Here we characterize a metal-dependent, bifunctional isoprenyl diphosphate synthase from the leaf beetle Phaedon cochleariae by structural and functional analyses. Isoprenyl diphosphate synthase in P. cochleariae (PcIDS1, EC 2.5.1.1) produces FPP in the presence of Mg2+, but preferably forms GPP when exposed to the heavy metal ions (HMIs) Co2+ or Mn2+. Inter- and intramolecular cooperative effects in the homodimer strongly depend on the provided metal ions and regulate the biosynthetic flux of terpene precursors to either biological defence or physiological development. Strikingly, a unique chain length determination domain adapts to form geranyl or farnesyl pyrophosphate by altering enzyme symmetry and ligand affinity between both subunits.

Stabilized by cation–π interactions with R427, the F315 side chain positions IPPHAl for nucleophilic attack. V286 and I420 form the bottom of this specificity pocket and act as a molecular ruler, whereas F282 and F315 engage in π-stacking with both allyl groups.

>[2x]GSFSKEESREFMAIFPDIVRDLTDAGRHTDIPEVTKRFAKVLQYNVPTGKKTRGLSTVIAYKMLEKPENLTPENVRLAGILGWCVELLQASLLIMDDLMDRSETRRGQPCWYRQENVGFLAINDCLHVESSLYSVLRKYFSHLPCYVPIIELFHDVNFKTNMGQSLDALCMKDGRPILSQFTMKRYSSIVKYKTSYYTFQLPVSLGMYLADMYDPEQHRQAKTILMEIGEFDQIQDDFLDAFGDSQVTGKVGTDIKEGKCSWLAVVALQRSNPAQRQIMEEHYGRPEPESTQIIKNLYIELGLPATFAVYEEESFNIIRTHIHQISKGLPHDLFFKIMKKIYKRDA> PTGLAADIRWTAYGVPHIRAKDERGLGYGIGYAYARDNACLLAEEIVTARGERARYFGSEGKSSAELDNLPSDIFYAWLNQPEALQAFWQ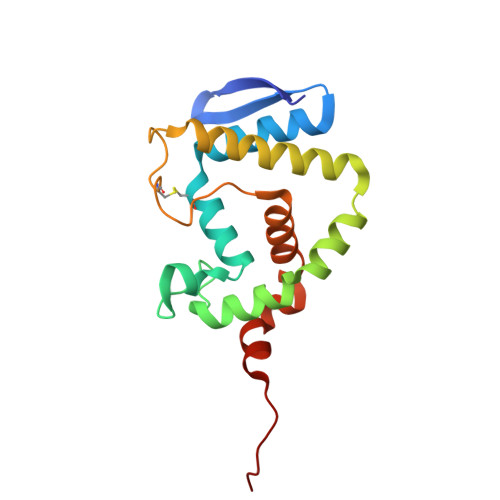AQTPAVRQLLEGYAAGFNRFLREADGKTTSCLGQPWLRAIATDDLLRLTRRLLVEGGVGQFADALVAAAPPGAEK> MNQANNVLDSIYQPDLEIMNQPEIELDDLLI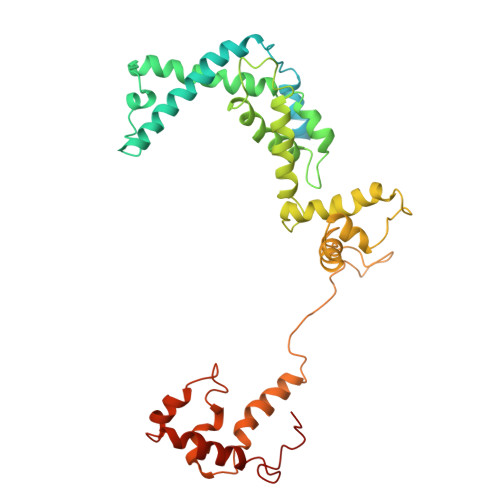EEDEDLLLADDGDIDEFLEPQTDEDDAKSGKAAKSRRRTQSKKKHYTEDSIRLYLQEIGRIRLLRADEEIELARKIADLLELERVRERLSEKLERDPRDSEWAEAVQLPLPAFRYRLHIGRRAKDKMVQSNLRLVVSIAKKYMNRGLSFQDLIQEGSLGLIRAAEKFDHEKGYKFSTYATWWIRQAITRAIADQSRTIRLPVHLYETISRIKKTTKLLSQEMGRKPTEEEIATRMEMTIEKLRFIAKSAQLPISLETPIGKEEDSRLGDFIESDGETPEDQVSKNLLREDLEKVLDSLSPRERDVLRLRYGLDDGRMKTLEEIGQIFNVTRERIRQIEAKALRKLRHPNRNSVLKEYIR>[2x]GTRKCELQGLWRNELGSNMTISALDVAGTFSGSYQTAVTATNKQILVSPLKGAQQPPGTKGQQPTFGFTVQWQFADSTTVFVGQCFVDRRGKEMLEMAWLLREEVPSRKDTWKATRVGTNVFTRVK

Here, we expand the repertoire of known macromolecular biotin binders by reporting a novel biotin-binding protein A (BBP-A) from chicken. In the present study, we show that the chicken BBP-A gene encodes a functional homotetrameric protein. The BBP-A structures consist of four identical subunits, each subunit adopting a β-barrel fold of eight anti-parallel β-strands with an α-helix positioned between the β7- and β8-strands. The BTN/BSO-binding site is located at the open end of each β-barrel.

We report two different X-ray structures of BBP-A, one in complex with BTN and an other one in complex with D-biotin D-sulfoxide (BSO), at 2.1 Å and 1.75 Å resolution, respectively. Surprisingly, in one of the two BBP-A crystals that were analyzed, BSO was found bound to BBP-A even though only BTN was added in the co-crystallisation experiments. To our knowledge, BSO is not found in any other protein structure presently within the Protein Data Bank (PDB). Electron density for the BSO ligand was clearly seen in the difference map of the BBP-A – BSO structure. The binding mode of BSO to BBP-A is surprisingly similar to that of BTN despite the additional oxygen atom that is covalently linked to the sulphur atom of the bicyclic ring system of BSO but is missing from BTN. The distance between the sulfur atom of BTN and the OG1 atom of Thr78 (3.4 Å), for example, is very close to the BSO – Thr78 distance (3.6 Å). The only noticeable difference around the ligands in the two BBP-A structures was found at Glu102, which in the BBP-A – BTN structure is hydrogen bonded to the valeric O10A atom of BTN but in the BBP-A – BSO structure was observed either to form a salt bridge with Arg115 (chains B and D) or to hydrogen bond to a structural water molecule (chains A and C). Moreover, in the BBP-A – BSO structure, the carboxylate side-chain of Glu102 forms a salt-bridge with the guanidinium group of the Arg115 side-chain within the same subunit (in chains B and D) or is hydrogen bonded to a structural water molecule (in chains A and C), interactions that are not seen in the BBP-A – BTN complex. Surprisingly, the affinity of BBP-A for BSO is even higher than the affinity for BTN. Of the three residues (Val116, Gly117 and Thr118) within 5 Å from each other at the 1–3 subunit interface of the BBP-A – BSO structure, valine and glycine are conserved between BBP-A and AVD, while Thr118 is replaced by Ile117 in the AVD structure.>MARDEVRRILPADIKREVIVKDDKAETNPKWGFPPDKRPI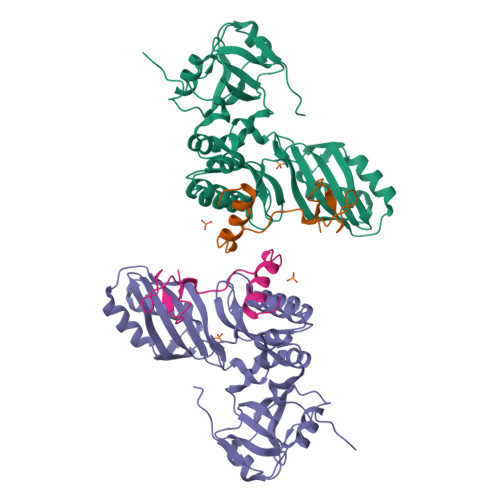ELHIQYGVINLDKPPGPTSHEVVAWIKRILNLEKAGHGGTLDPKVSGVLPVALERATRVVQALLPAGKEYVALMHLHGDVPEDKIRAVMKEFEGEIIQRPPLRSAVKRRLRTRKVYYIEILEIDGRDVLFRVGVEAGTYIRSLIHHIGLALGVGAHMAELRRTRSGPFKEDETLVTLHDLVDYYHFWKEDGIEEYIRKAIQPMEKAVEHLPKIWIKDSAVAAVAHGANLTVPGIVKLNAGIKKGDLVAIMTLKDELVALGKAMMSTQEMIERSKGIAVDVEKVFMPRDWYPKLW[2x];>[2x]MRFRIRKCPKCGRYTLKETCPVCGEKTKVAHPPRFSPEDPYGEYRRRLKRELLGIGRKEK4-amino-3-hydroxy-9,10-dioxo-9,10-dihydroanthracene-2-sulfonic 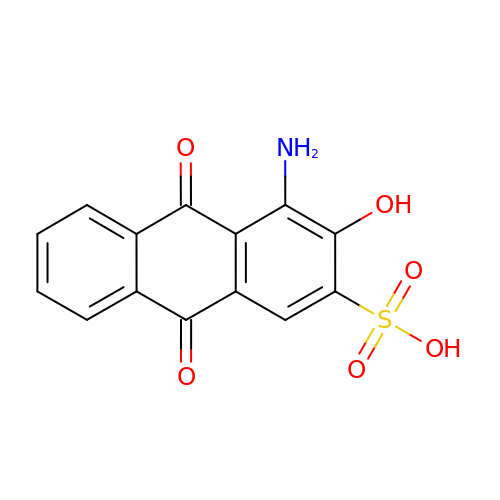acid | C14 H9 N O6 S | CDACXRLIDPHNCR-UHFFFAOYSA-N> QPQFNEDTLQQRLQALIESAGENWTYAIFWQISHDFDSSTGDNTVILGWGDGYYKGEEDKEKKKNNTNTAEQEHRKRVIRELNSLISGGIGVSDESNDEEVTDTEWFFLVSMTQSFVNGVGLPGESFLNSRVIWLSGSGALTGSGCERAGQGQIYGLKTMVCIATQ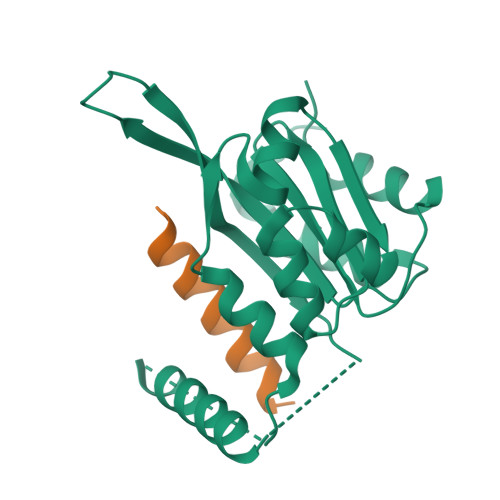NGVVELGSSEVISQSSDLMHKVNNLFNFN;> SVPQARKASLARFLEKRKERLM>MKVIFLKDVKGMGKKGEIKNVADGYANNFLFKQGLAIEA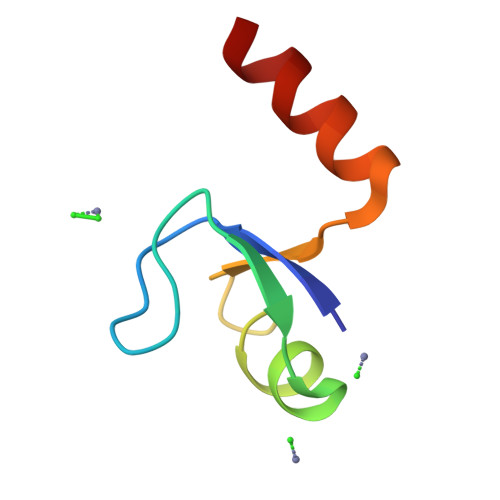TPANLKALEAQKQ[2x]> SSGQISIQPTFS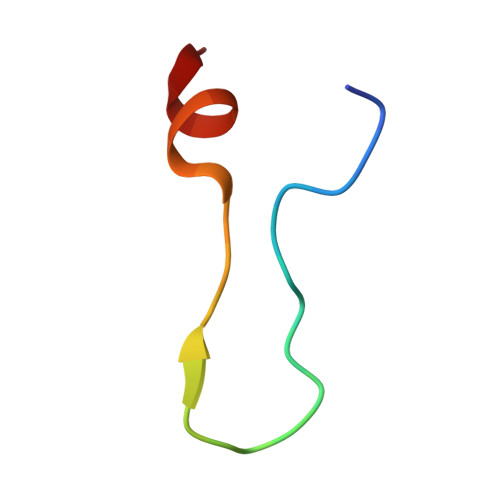VQRNLPFDRPTIMAA> MGSSHHHHHHSQDPMGQVLPLVTRQGDRIAIVSGLRTPFARQATAFHGIPAVDLGKMVVGELLARSEIPAEVIEQLVFGQVVQMPEAPNIAREIVLGTGMNVHTDAYSVSRACATSFQAVANVAESLMAGTIRAGIAGGADSSSVLPIGVSKKLARVLVDVNKARTMSQRLKLFSRLRLRDLMPVPPAVAEYSTGLRMGDTAEQMAKTYGITREQQDALAHRSHQRAAQAWSDGKLKEEVMTAFIPPYKQPLVEDNNIRGNSSLADYAKLRPAFDRKHGTVTAANSTPLTDGAAAVILMTESRAKELGLVPLGYLRSYA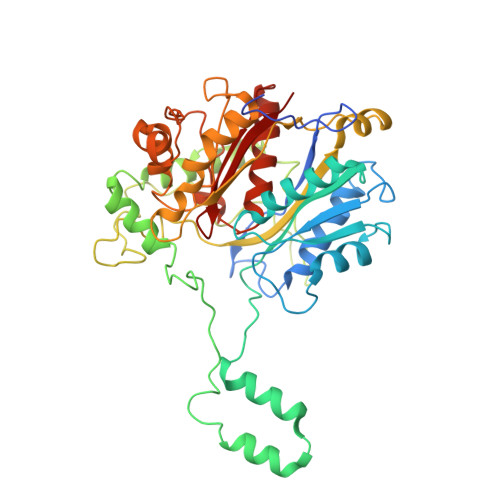FTAIDVWQDMLLGPAWSTPLALERAGLTMSDLTLIDMHEAFAAQTLANIQLLGSERFAREALGRAHATGEVDDSKFNVLGGSIAYGHPFAATGARMITQTLHELRRRGGGFGLVTACAAGGLGAAMVLEAE>[8x]M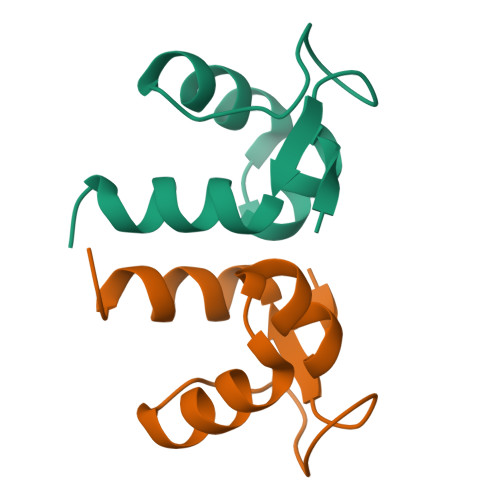NVNKKKLAEIFGCDVRTVTAWQSQGLPLVSGGGKGNEAVFDTAAAISWYAERDA>GERPYMQPFHLIPPSLSVQATEQPLASNEAWDYPEPLAPGQSPAASSEEGSSEEKGDEREPHGDEGKRGRKDKKKSKTQRIASAVNGLGFRLYKQVLGGAGPADNIFFSPLSIASALGVVTAGANGSTRAELDTALGFKEFLHGKKKAKSMKYFARLNGALYKRSAGFELMGKNVVFSKKGLWLYRQFTRTVAHLFKSNVRSVDFGDSKNAVELMNAYIEKVTSKKFPDVISDVDTDTSLVIVNVIYFKGSWGNKFEPDLTKNVRFWVNSSYSMMVPTMHQRAKLSYTQD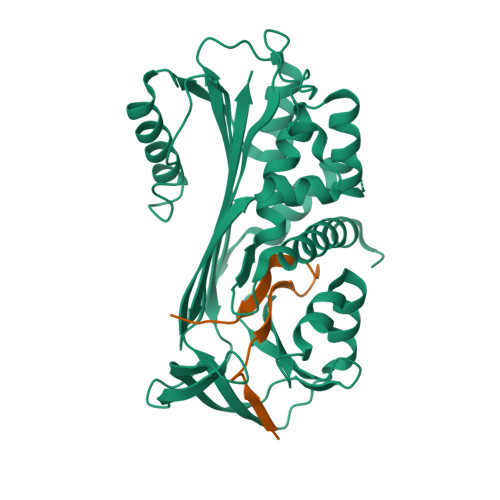RKLRSTVVKLPYEGGASMLVIVPHRTEDLPKVEESVSQEQLEEWLSLLGPSNHYVQLSLPKFKISVSYDLKAYLSAMGMSSMFSYGADLSRITGMQKLHVDKITHKSVLHVNEEGTEAKAETVVGIMAAPR[2x];>[2x]SMPPTVTVDRPFVVLIYDEKTRAVIFMGRVADPKQ> MTDKLIRELLIDVKQKGATRTAKSIENVSDALENAAAASELTNEQLGKMPRTLYSIERAADRAAKSLTKMQASRGMAGITKSIDGIGDKLDYLAIQLIEVTDKLEIGFDGVSRSVKAMGNDVAAATEKVQDRLYDTNRALGGTSKGFNDTAGAAGRASRALGNTSGSARGATRDFAAMAKIGGRLPIMYAALASNVFVLQTAFESLKVGDQLNRLEQFGTIVGTMTGTPVQTLALSLQNATNGAISFEEAMRQASSASAYGFDSEQLEQFGLVARRAAAVLGVDMTDALNRVIKGVSKQEIELLDELGVTIRLNDAYEN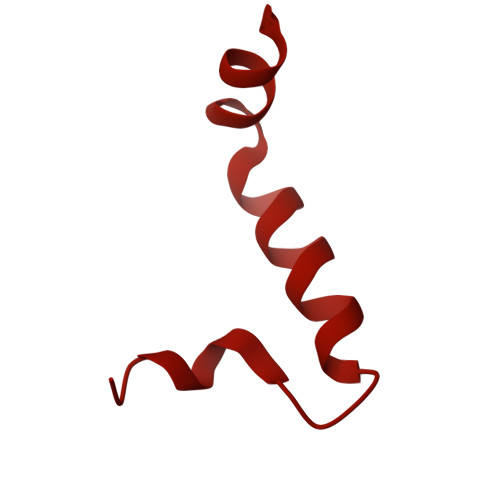YVKQLNATSTGIKYTVDSLTTYQKQQAYANEVIAESTRRFGYLDDALKATSWEQFAANANSALRSLQQSAATYLNPVMDTLNTFLYQTKSSQMRVSAMARSASAKTTPAENVTALIENAVGAREDLDTYLKESEERVKKAQELKQQLDDLKAKQAATAPIANALTAGGIGGDESNKLVVQLTNELARQNKEIEERTKTEKVLRQAVQDTGEALLRNGKLAEQLGAKMKYADTAVPGDKGVFEVDPNNLKAVSEIQKNFDFLKKSSSDTANNIRMAASSITNAKKASSDLNSVVKAVEDTSKVTGQSADTLVKNLNLGFSSLDQMKAAQKGLSEYVTAMDKSEQNALEVAKRKDEVYNQTKDKAKAEAAAREVLLRQQQEQLTAAKALLAINPNDPEALKQVAKIETEILNTKAQGFENAKKTKDYTDKILGVDREIALLNDRTMTSTQYRLAQLRLELQLEQEKTELYSKQADGQAKVEQSRRAQAQISREIWEAEKQGTASHVSALMDALEVSQTQRNVTGQSQILTERLSILQQQLELSKGNTEEELKYRNEIYKTSAALEQLKKQRESQMQQQVGSSVGATYTSTTGLIGEDKDFADMQNRMASYDQAISKLSELNSEATAVAQSMGNLTNAMIQFSQGSLDTTSMIASGMQTVASMIQYSTSQQVSAIDQAIAAEQKRDGKSEASKAKLKKLEAEKLKIQQDAAKKQIIIQTAVAVMQAATAVPYPFSIPLMVAAGLAGALALAQASSASGMSSIADSGADTTQYLTLGERQKNVDVSMQASSGELSYLRGDKGIGNANSFVPRAEGGMMYPGVSYQMGEHGTEVVTPMVPMKATPNDQLSDGSKTTSGRPIILNISTMDAASFRDFASNNSTAFRDAVELALNENGTTLKSLGNS ACMSD, the enzyme responsible for decarboxylating α-amino-β-carboxymuconate-ε-semialdehyde (ACMS) to produce α-aminomuconate-ε-semialdehyde (2-AMS), plays a crucial role in controlling QUIN levels. This zinc-dependent metalloprotein is situated within the tryptophan-kynurenine pathway, where it competes with a spontaneous chemical reaction that converts ACMS directly to QUIN. With the cavity of ACMSD, a mononuclear Zn2+ ion coordinates with His9, His11, His177, Asp294, and a water molecule (residue numbering based on ACMSD from Pseudomonas fluorescens, pfACMSD). ACMSD functions as a dimer, with residue Arg239∗ from the adjacent subunit being crucial for the decarboxylation reaction.

Trp194, located approximately 5 Å away from the Zn ion, possesses a bulky side chain in the active site of the ligand-free structure, suggesting its potential participation in the ACMS decarboxylation. Here, we replaced Trp194 with alanine to examine its role in catalysis. The crystal structure of W194A was determined at the resolution of 2.02 Å. W194A maintains the overall structure of ACMSD, with an RMSD value of 0.265 Å on 265 Cα. Comparative analysis revealed that mutants H228A and W194A exhibit a significant decrease in kcat values for ACMS decarboxylation by 142-fold and 26-fold, respectively, relative to wild-type ACMSD, indicating the essential roles of His228 and Trp194 in ACMS decarboxylation. The 1.9-fold increase in KM value for W194A suggests a minimal role in substrate binding, potentially shielding the active site from the solvent. Interestingly, mutating His228 to Tyr abolishes the tautomerization activity, while H228A and W194A mutants exhibit comparable kcat and KM values to wild-type ACMSD. These findings indicate that His228 and Trp194 are not involved in catalyzing OAA tautomerization. Subsequently, a nearby base deprotonates the C3 carbon, while an acid protonates the carbonyl oxygen of the keto form of OAA, resulting in the production of its enol form as the product. Despite the structural proximity of Trp194 and His228 to the active site, they are unlikely to be the base, as demonstrated by the comparable tautomerization activity of H228A and W194A mutants compared to the wild-type ACMSD.

>[3x]MKKPRIDMHSHFFPRISEQEAAKFDANHAPWLQVSAKGDTGSIMMGKNNFRPVYQALWDPAFRIEEMDAQGVDVQVTCATPVMFGYTWEANKAAQWAERMNDFALEFAAHNPQRIKVLAQVPLQDLDLACKEASRAVAAGHLGIQIGNHLGDKDLDDATLEAFLTHCANEDIPILVHPWDMMGGQRMKKWMLPALVAMPAETQLAILSLILSGAFERIPKSLKICFGHGGGSFAFLLGRVDNAWRHRDIVREDCPRPPSEYVDRFFVDSAVFNPGALELLVSVMGEDRVMLGSDYPFPLGEQKIGGLVLSSNLGESAKDKIISGNASKFFNINV2-[(5-BROMO-2-PYRIDYL)-METHYL-AMINO]ETHANOL | C8 H11 Br N2 O | 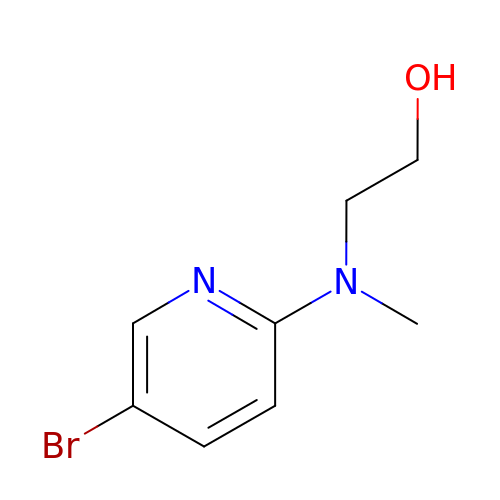FWDPWBASDJULOB-UHFFFAOYSA-N>[4x]ADVTITVNGKVVAKP;>[4x]FACKTANGTAIPIGGGSANVYVNLAPAVNVGQNLVVDLSTQIFCHNDYPETITDYVTLQRGSAYGGVLSSFSGTVKYNGSSYPFPTTSETPRVVYNSRTDKPWPVALYLTPVSSAGGVAIKAGSLIAVLILRQTNNYNSDDFQFVWNIYANNDVVVPTGGCDVSARDVTVTLPDYPGSVPIPLTVYCAKSQNLGYYLSGTTADAGNSIFTNTASFSPAQGVGVQ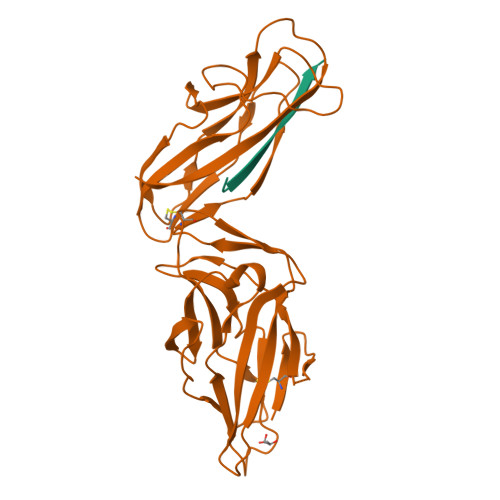LTRNGTIIPANNTVSLGAVGTSAVSLGLTANYARTGGQVTAGNVQSIIGVTFVYQ>[2x]APSRKFFVGGNWKMNGRKQSLGELIGTLNAAKVPADTEVVCAPPTAYIDFARQKLDPKIAVAAQNCYKVTDGAFTGEISPGMIKDCGATWVVLGHSERRHVFGESDELIGQKVAHAL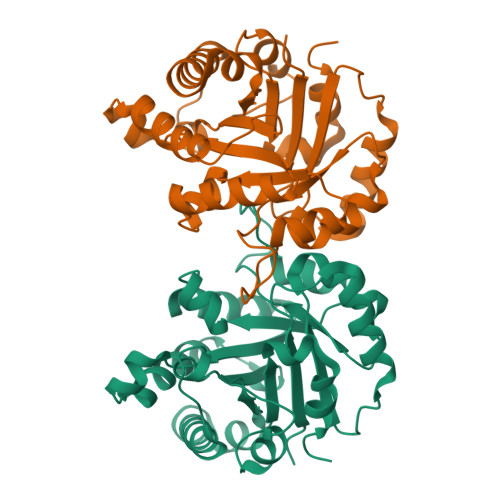AEGLGVIACIGEKLDEREAGITEKVVFEQTKVIADNVKDWSKVVLAYEPVWAIGTGKTATPQQAQEVHEKLRGWLKSNVSDAVAQSTRIIYGGSVTGATCKELASQPDVDGFLVGGASLKPEFVDIINAKQ>[2x]VMKRVAIFASGSGTNAEAIIQSQKAGQLPCEVALLITDKPGAKVVERVKVHEIPVCALDPKTYPSKEAYEIEVVQQLKEKQIDFVVLAGYMRLVGPTLLGAYEG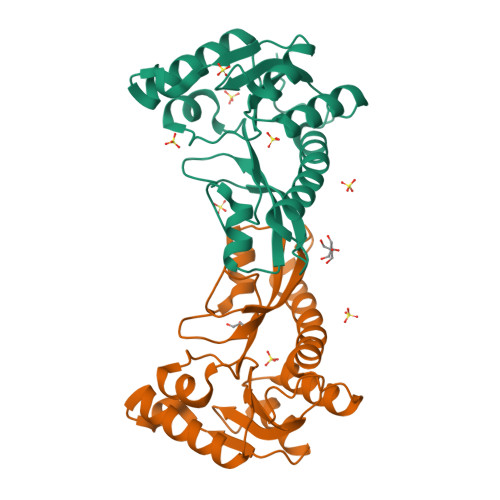RIVNIHPSLLPAFPGLHAIEQAIRANVKVTGVTIHYVDEGMDTGPIIAQEAVSIEEEDTLETLTTKIQAVEHRLYPATLHKLLSKAENLYFQSHHHHHHWSHPQFEK>[7x]MTEPKFKGLRLELAVDKMVTCIAVGLPLLLISLAFAQEISIGTQISCFSPSSFSWRQAAFVDSYCWAAVQQKNSLQSESGNLPLWLHKFFPYILLLFAILLYLPPLFWRFAAAPHICSDLKFIMEELDKVYNRAIKAAKSARDLDMRDGACSVPGVTENLGQSLWEVSESHFKYPIVEQYLKTKKNSNNLIIKYISCRLLTLIIILLACIYLGYYFSLSSLSDEFVCSIKSGILRNDSTVPD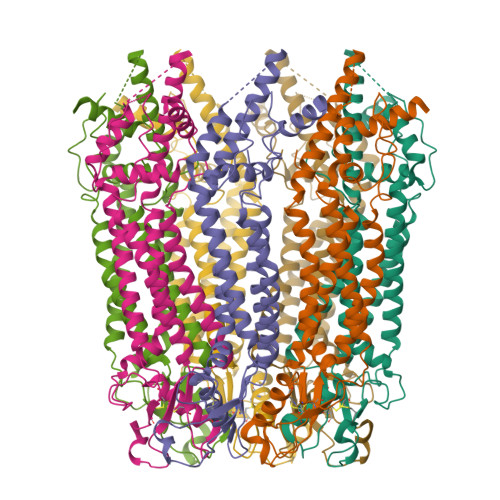QFQCKLIAVGIFQLLSVINLVVYVLLAPVVVYTLFVPFRQKTDVLKVYEILPTFDVLHFKSEGYNDLSLYNLFLEENISEVKSYKCLKVLENIKSSGQGIDPMLLLTNLGMIKMDVVDGKTPMSAEMREEQGNQTAELQGMNIDSETKANNGEKNARQRLLDSSC> GLGQMGSSSTDNTVRETVGAATSRDALPNTEASGPTHSKEIPALTAVETGATNPLVPSDTVQTRHVVQHRSRSESSIESFFARGACVTIMTVDNPASTTNKDKLFA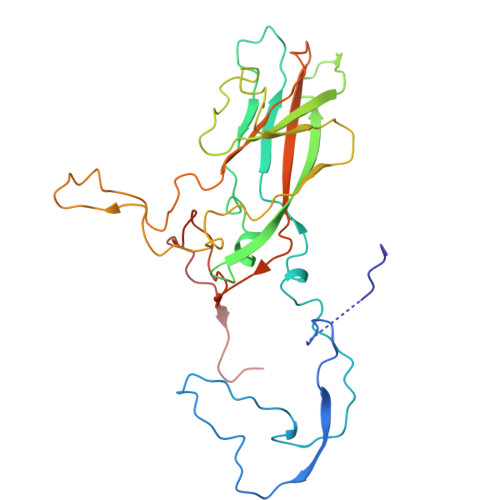VWKITYKDTVQLRRKLEFFTYSRFDMELTFVVTANFTETNNGHALNQVYQIMYVPPGAPVPEKWDDYTWQTSSNPSIFYTYGTAPARISVPYVGISNAYSHFYDGFSKVPLKDQSAALGDSLYGAASLNDFGILAVRVVNDHNPTKVTSKIRVYLKPKHIRVWCPRPPRAVAYYGPGVDYKDGTLTPLSTKDLTTY> DEAAELMQQVNVLKLTVEDLEKERDFYFGKLRN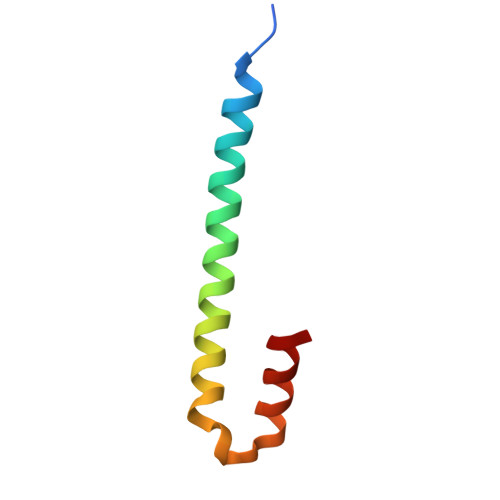IELICQENEGENDPVLQRIVDILYA>HMIHEDFCSVCRKSGQLLMCDTCSRVYHLDCLDPPLKTIPKGMWICPRCQDQMLKKEEAI[2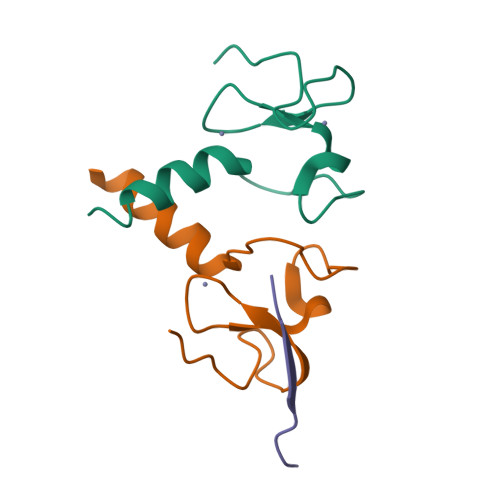x];> ARTKQTARKS>[6x]SNAMTTYTSIANVIKERRSVRTFTDKAVEKDLLIELLNDATWAPNHKHREPWNCKLYIGEGRKKLVDAVLNSFTEEERAKRGKILSDRFLSTPAQIVVYMNEDPRQIQRDE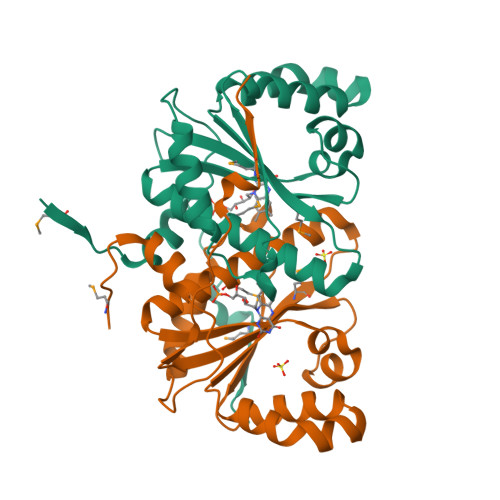DYAATCAFMQNFQLLAWERGLGCVWKSGGLNYNPLFIEGIGLTRGQRIVGILHIGYFDKAPEGKARTPITEKMEIIEG>[2x]GSMLTIGQLARIFEISTKTLRHYDAIGLFVPARTGSDNGYRYYQPEQIEQLSRILALRRLDVPLEAIDRLKRDGA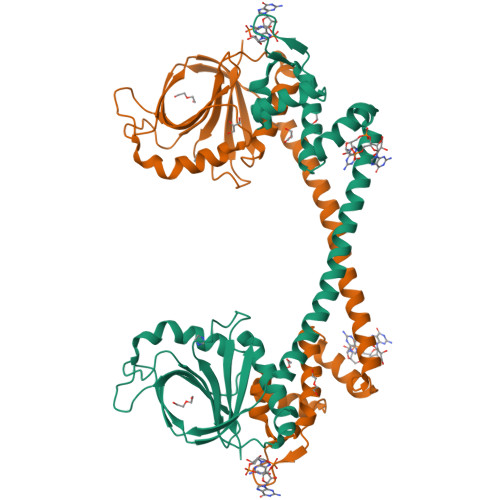LDDPQRLRHFLQRHQHTLREEISARQRLLAELDRTLATLAHWRIRNMHARIVERPAFSVVGMEYFGSAPGDTIGQLWERFIPREHEIAGKHDPEVSYGICAQQPNGEFHYVAGFEVQEGWPVPEGMVRFQVPAQKYAVFTHKGTAPQIAESFQAIYSHLLAERGLEPKAGVDFEYYDQRFRGPLDPNSQVDLYIPIY>LDNGLARTPTMGWLHWERFMCNLDCQEEPDSCISEKLFMEMAELMVSEGWKDAGYEYLCIDDCWMAPQRDSEGRLQADPQRFPHGIRQLANYVHSKGLKLGIYADVGNKTCAGFPGSFGYYDIDAQTFADWGVDLLKFAGCYCDSLENLADGYKHMSLALNRTGRSIVYSCEWPLYMWPFQKPNYTEIRQYCNHWRNFADIDDSWKSIKSILDWTSFNQERIVDVAGPGGWNDPDMLVIGNFGLSWNQQVTQMALWAIMAAPLFMSNDLRHISPQAKALLQDKDVIAINQDPLGKQGYQLRQGDNFEVWERPLSGLAWAVAMINRQEIGGPRSYTIAVASLGKGVACNPACFITQLLPVKRKLGFYEWTSRLRSHINPTGTVLLQLENTMQMSLKDLLDYKDDDDKDYKDDDDK[2x];> GASGDVCQDCIQMVTDIQTAVRTNSTFVQALVEHVKEECDRLGPGMADICKNYISQYSEIAIQMMMHMQPKEICALVGFCDE

Four mature saposins (SapA, SapB, SapC, and SapD) result from proteolysis of the precursor prosaposin as it traffics to the lysosome. The saposin family members are disulfide-linked, four-helix bundles that usually form dimers. SapB presents a variety of ligands to several lysosomal hydrolases, including arylsulfatase A, β-galactosidase (GLB1), and α-galactosidase A (GLA). One cargo, globotriaosylceramide (Gb3), is presented exclusively by SapB to GLA for removal of the terminal α-galactose, and failure of this process leads to accumulation of Gb3 in the lysosome and ultimately results in Fabry disease.

While crystals of SapB:GLA complexes did not readily form in the presence of the lipid, we did isolate diffraction-quality crystals of a SapB:GLA complex in the presence of DDAO detergent. We determined the structure of SapB bound to GLA at 3.53 Å resolution. The structure of SapB bound to GLA contains a dimer of GLA and monomer of SapB in the asymmetric unit. However, the SapB monomer lies on a crystallographic two-fold axis, generating a symmetry-related SapB pair of monomers resting in the concave architecture of a pair of GLA dimers. The SapB pair is proximal to all four active sites of GLA, and the two SapB monomers do not contact each other. One SapB monomer rests asymmetrically across the GLA homodimer, contacting each of the two domains of a GLA monomer. The interacting residues between SapB and GLA at the dimer interface of GLA show charge complementarity, particularly involving the region surrounding the loop between the α3 and α4 helices of SapB. The complex interface contains backbone and side-chain hydrogen bonds and salt bridges, involving Asp231, Asp233, Lys237, Lys240, and Asp244 on GLA and Arg19, His64, Gln66, and Glu69 on SapB. In contrast, the hairpin of SapB, which lies near the active site disulfide bond (Cys142-Cys172) of GLA, interacts largely via van der Waals interactions, with one hydrogen bond between Pro41 on SapB and Tyr173 on GLA. We aligned the SapB:Gb3-NBD structure to SapB in the GLA complex. This alignment demonstrated that both a 14° narrowing of the SapB hinge angle and a 19 Å separation of the SapB dimer were necessary to form the SapB pair in the SapB:GLA crystal.> QDADKLPHTKVTLVAPPQVHPHEQATKSGPKVVEFTMTIEEKKMVIDDKGTTLQAMTFNGSMPGPTLVVHEGDYVQLTLVNPATNAMPHNVDFHGATGALGGAKLTNVNPGEQATLRFKADRSGTFVYHCAPEGMVPHHVVSGMSGTLMVLPRDGLKDPQGKPLHYDRAYTIGEFDLYIPKGPDGKYKDYATLAESYGDTVQVMRTLTPS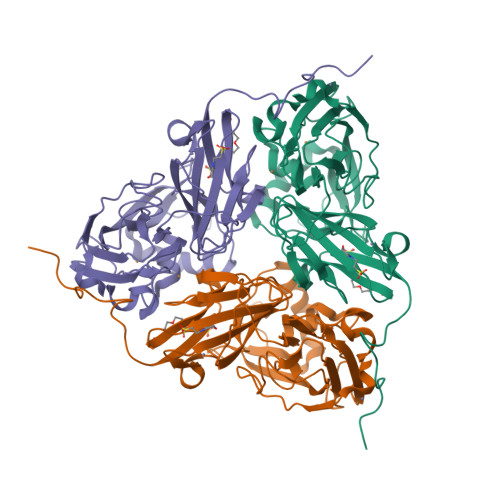HIVFNGKVGALTGANALTAKVGETVLLIHSQANRDTRPHLIGGHGDWVWETGKFANPPQRDLETWFIRGGSAGAALYTFKQPGVYAYLNHNLIEAFELGAAGHIKVEGKWNDDLMKQIKAPAPIPR GEN1 is a member of a superfamily of structure-selective nucleases (Grasby et al., 2012). The structure of the GEN1 protein reveals it to have an elaborated FEN-XPG family fold that is modified for its role in four-way junction resolution. In free solution the protein exists primarily in monomeric form, but binds to DNA junctions as a discrete dimer to generate bilateral cleavage by accelerating second strand cleavage. We have now solved a crystal structure of active GEN1 from C. thermophilum bound to the DNA resulting as the product of cleavage.

The crystals belong to the P3121 space group, in which the asymmetric unit contains one CtGEN1 monomer and a duplex of DNA with 14 and 15 nt strands (14 bp with a 3′ overhang) that adopts a standard B-form helix with no distortion. The cavity contains six conserved acidic amino acids, contributed by the N-terminal ends of α6, α7, and the C-terminal ends of β2 and β3. Metal ions are bound in the middle of this cluster of acidic side chains. For the original Mg2+ crystals, a single bound ion (M2) was observed, but after soaking the crystals with MnCl2, two bound metal ions were observed. (B) After exposure of the crystal to Mn2+ ions, two bound metal ions are observed. These are coordinated to the six carboxylate side chains and the terminal phosphate group (P5′). Metal ion M2 is 2.1 Å from the carboxylate groups of D141 and D143, while M1 is 2.2 Å from the carboxylate group of E122, 4.1 Å from that of D38 and D79, and 4.7 Å from E120. Moreover, the position of the 5′-terminal phosphate relative to the two metal ions in the cleavage site in the product complex is not suitable for in-line attack by a metal-bound water molecule, so the geometry in the active site must have rearranged after cleavage. It is also very probable that the metal ions have moved from their positions prior to the cleavage reaction.

> GIKGIYKEIGSGERISLCKLAIDHLEQHNRPLRLAIDMAIWQFQIQAARGGSNPAIRTLFYRFVRLLSLGIHPIFVFDGPNKPIFKRNRRSGTGNGVSTAMAKRLIRLFGFTAHDAPGEAEAECAYLEQQGIVDAVLSEDVDTIMFGSRVTLRDWSSEGSKGGPPTHVTLHDAKKIAEGPSGLDREGMVLVALMSGGDYLPDGIPGCGIKVACQAAKAGFGKELCRIKRADKEAITEWKQRLLHELRTNESGFFRTKHKALEIPENFPNMEVLRYYTHPVVSSPATIERLRQEFPPSSTVDIAGLREFTRETFDWTFRPGAIKLIKVLAPGLLVQRCLDRYVSGPRIDDPDLKKKEESTLVKGISMRREHFSTDATPELRVSFIPAELVGLDPGQEPEVQVEAFGRSGLALNSDDEFDEDISSSQKAPKKPFDPWQPDLAWVPETILKLGVPVTVEDWEEGQRS>GAMDMETPSQRRATRSGAQASSTPLSPTRITRLQEKEDLQELNDRLAVYIDRVRSLETENAGLRLRITESEEVVSREVSGIKAAYEAELGDARKTLDSVAKERARLQLELSKVREEFKELKARNTKKEGDLIAAQARLKDLEALLNSKEAALSTALSEKRTLEGELHDLRGQVAKLEAALGEAKKQLQDEMLRRVDAENRLQTMKEELDFQKNIYSEELRETKRRHETRLVEIDNGKQREFESRLADALQELRAQHEDQVEQYKKELEKTYSAKLDNARQSAERNSNLVGAAHEELQQSRIRID[4x]

Intermediate filament (IF) proteins form flexible fibrous structures that provide vital mechanical support in higher eukaryotic cells. Nuclear lamins are IF proteins that play an essential role in maintaining the nuclear envelope structure. They have been implicated in diverse cellular processes, including mitosis, chromatin organization, DNA replication, and transcription. The lamin filaments make up the three-dimensional meshwork underlying the inner nuclear envelope.

We determined the crystal structure of an N-terminal half fragment of human lamin A/C (residues 1–300; referred to as ‘lamin 300 fragment’ in this study) at a resolution of 3.2 Å. This spans the N-terminal head, coil 1a, L1, coil 1b, L12, and the first half of coil 2. The asymmetric unit consists of four protomers (chains A–D), which are bundled by an anti-parallel pair of parallel helical dimers (chain A:B and C:D). A typical left-handed coiled-coil conformation was found in most of the coil 1a and the N-terminal four-fifths of coil 1b, in which hydrophobic residues were regularly found at the heptad positions a and d (highlighted in yellow). Linker L1 and an adjacent coil 1b segment (residues 70–84) showed the hendecad pattern, which induces the formation of an untwisted helical section. In the helical dimers, coil 1b consists of the 18 N-terminal heptad repeats (residues 79–204) forming a left-handed coiled-coil structure (~22 nm; one and a half super-helical turn) and the two C-terminal hendecad repeats (residues 204–222) forming an untwisted helical section. The hendecad repeat region in coil 1b is continuous to the N-terminal half of L12 (residues 223–230), unlike previous predictions proposing a flexible hinge conformation. The untwisted helical section is bent asymmetrically near the junction between L12 and coil 2, leading to mismatched inter-helical hydrophobic interactions. Coil 1b and its flanking linker segments (residues 67–221) form the anti-parallel contacts between coiled-coil dimers, and the remaining parts (coil 1a and coil 2) are bifurcated from both sides of the contacting region. From these observations, we concluded that the anti-parallel interaction between the two coiled-coil dimers in the asymmetric unit of lamin corresponds to the ‘A11 interaction’ of vimentin18,33–35.> MSSRNNPARVAIVMGSKSDWATMQFAAEIFEILNVPHHVEVVSANRTPDKLFSFAESAEENGYQVIIAGAGGAAHLPGMIAAKTLVPVLGVPVQSAALSGVDSLYSIVQMPRGI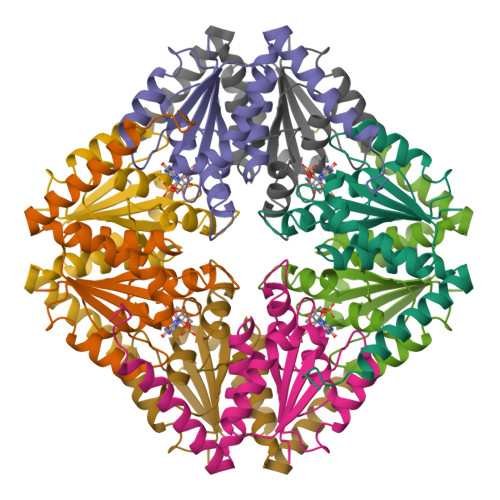PVGTLAIGKAGAANAALLAAQILATHDKELHQRLNDWRKAQTDEVLENPDPRGAA The NAD(P)+-dependent succinate semialdehyde dehydrogenase (SSADH) Sad is a member of the ALDH superfamily and oxidizes succinate semialdehyde (SSA) to succinate. In microorganisms, SSADHs operate in the degradation of various nitrogen-containing compounds such as putrescine or arginine, where they prevent the accumulation of the toxic SSA intermediate. Our results show that Sad is a surprisingly flexible enzyme that is not only able to detoxify succinate semialdehyde and glutarate semialdehyde but can also functionally substitute erythrose 4-phosphate dehydrogenase in pyridoxal 5′-phosphate (PLP) biosynthesis and glyceraldehyde 3-phosphate dehydrogenase (as well as phosphoglycerate kinase) in glycolysis under physiological conditions. We show that Sad, which primarily functions in the detoxification of succinate semialdehyde in various degradation pathways, does not only accept closely related substrates, but also converts phosphorylated sugars as a side reactivity.

To understand the molecular basis of the improved enzyme activity in the Q262R variant, we solved the crystal structures of both Sad WT and Q262R variants with bound NAD+, as well as in complex with both NAD+ and SSA. Two-tailed t-test, P-values are shown, and error bars represent SD. e The active site of the wild-type Sad with bound NAD+ (dark gray) and substrate (salmon) SSA, the latter is covalently bound to C268. We next purified the WT and Q262R variants of Sad for biochemical characterization. Both enzymes possessed high activity with SSA (~90 μmol min−1 mg−1), the native substrate, which was unchanged for the Q262R variant compared to the WT. Even more surprisingly, when testing the substrate spectrum of Sad, we noticed that the WT enzyme was able to directly accept E4P, notably at four-fold higher activity (50 nmol min−1 mg−1) compared to D-erythrose. Moreover, in the Q262R variant, E4P dehydrogenase activity was increased 17-fold compared to the WT, reaching 800 nmol min−1 mg−1. Both variants were also active with glyceraldehyde 3-phosphate (GAP), showing even higher activities with GAP compared to E4P. While we were not able to obtain structures with sufficient electron densities for the alternative sugar-phosphate substrates, we manually fitted E4P and GAP based on the NAD+/SSA-bound structures. We hypothesized that this increase in gene dose resulted in increased intracellular Sad activity so that Sad could also oxidize sufficient E4P in vivo. This was in line with our biochemical characterization of Sad, which had shown that the WT enzyme already exhibited physiologically relevant kinetic parameters with E4P, in particular an app.

>[4x]MTITPATHAISINPATGEQLSVLPWAGADDIENALQLAAAGFRDWRETNIDYRAEKLRDIGKALRARSEEMAQMITREMGKPINQARAEVAKSANLCDWYAEHGPAMLKAEPTLVENQQAVIEYRPLGTILAIMPWNFPLWQVMRGAVPIILAGNGYLLKHAPNVMGCAQLIAQVFKDAGIPQGVYGWLNADNDGVSQMIKDSRIAAVTVTGSVRAGAAIGAQAGAALKKCVLELGGSDPFIVLNDADLELAVKAAVAGRYQNTGQVCAAAKRFIIEEGIASAFTERFVAAAAALKMGDPRDEENALGPMARFDLRDELHHQVEKTLAQGARLLLGGEKMAGAGNYYPPTVLANVTPEMTAFREEMFGPVAAITIAKDAEHALELANDSEFGLSATIFTTDETQARQMAARLECGGVFINGYCASDARVAFGGVKKSGFGRELSHFGLHEFCNIQTVWKDRI> GLGDLIEGVVEGVTRNALTPLTPANNLPDTQSSGPAHSKETPALTAVETGATNPLVPSDTVQTRHVIQKRTRSESTVESFFARGACVAIIEVDNDAPTKRASKLFSVWKITYKDTVQLRRKLEFFTYSRFDMEFTFVVTSNYTDANNGHALNQVYQIMYIPPGAPIPGKWNDYTWQTSSNPSVFYTYGAPPARISVPYVGIANAYSHFYDGFAKVPLAGQASTEGDSLYGAASLNDFGSLAVRVVNDHNPTKLTSKIRVYMKPKHVRVWCPRPPRAVPYYGPGVDYKDGLAPLPEKGLTTY;> MGAQVSSQKVGAHENSNRAYGGSTINYTTINYYRDSASNAASKQDFAQDPSKFTEPIKDVLIKTAPTLNSPNIEACGYSDRVMQLTLGN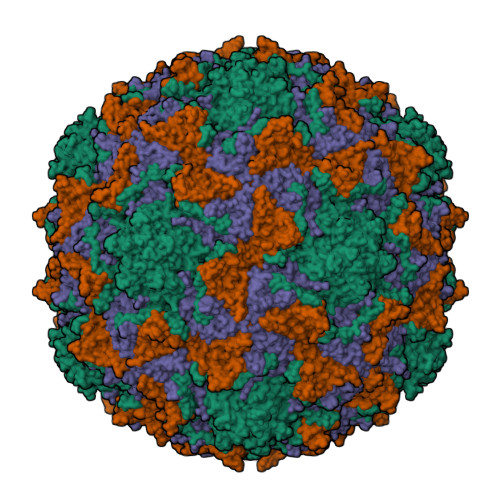STITTQEAANSVVAYGRWPEYIKDSEANPVDQPTEPDVAACRFYTLDTVTWRKESRGWWWKLPDALKDMGLFGQNMFYHYLGRAGYTVHVQCNASKFHQGALGVFAVPEMCLAGDSTTHMFTKYENANPGEKGGEFKGSFTLDTNATNPARNFCPVDYLFGSGVLAGNAFVYPHQIINLRTNNCATLVLPYVNSLSIDSMTKHNNWGIAILPLAPLDFATESSTEIPITLTIAPMCCEFNGLRNITVPRTQ;> GLPVLNTPGSNQYLTADNYQSPCAIPEFDVTPPIDIPGEVRNMMELAEIDTMIPLNLTNQRKNTMDMYRVELNDAAHSDTPILCLSLSPASDPRLAHTMLGEILNYYTHWAGSLKFTFLFCGSMMATGKLLVSYAPPGAEAPKSRKEAMLGTHVIWDIGLQSSCTMVVPWISNTTYRQTINDSFTEGGYISMFYQTRVVVPLSTPRKMDILGFVSACNDFSVRLLRDTTHISQEAMPQ> SMGEIESYCNKELGPLPTKAPTLSKNVLDLFSLKGKVASVTGSSGGIGWAVAEAYAQ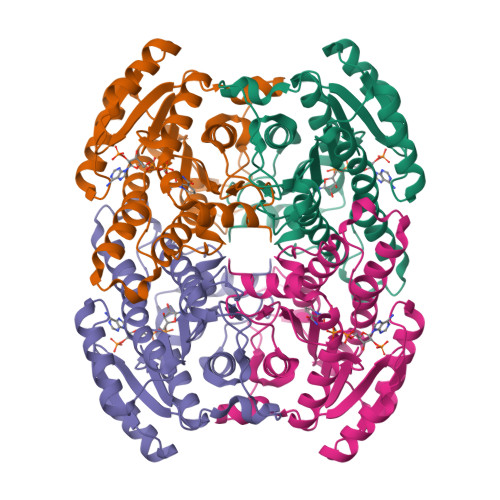AGADVAIWYNSHPADEKAEHLQKTYGVHSKAYKCNISDPKSVEETISQQEKDFGTIDVFVANAGVTWTQGPEIDVDNYDSWNKIISVDLNGVYYCSHNIGKIFKKNGKGSLIITSSISGKIVNIPQLQAPYNTAKAACTHLAKSLAIEWAPFARVNTISPGYIDTDITDFASKDMKAKWWQLTPLGREGLTQELVGGYLYLASNASTFTTGSDVVIDGGYTCP;> SMGEIESYCNKELGPLPTKAPTLSKNVLDLFSLKGKVASVTGSSGGIGWAVAEAYAQAGADVAIWYNSHPADEKAEHLQKTYGVRSKAYKCNISDPKSVEETISQQEKDFGTIDVFVANAGVPWTEGPEINVDNYDSWNKIINLDLNGVYYCAHTVGKIFKKNGKGSLVITSSMSGTIVNVPQLQAAYNAAKAACTHLTKSLAVEWAPFARVNCVSPGYIATEISDFVEKDMKAKWWQLTPLGREGLAQELVGAYLYLASNASTYTTGANLAVDGGYTCP>MKTRLEQVLERYLNGREVAVWGVPTRRLLRALKPFKFHTADRVDPQYHYVVAVTDDDLTDFLSDEQSKSFQYANDYLTFDDEGGELPFERMCFNVPVGRQTYFGDGVVGACENGYIKSIGQFTSINGTAEIHANHQLNMTFVSDDIQNFFNEESMAVFQEKLRKDPKHPYAYSKEPMTIGSDVYIGAHAFINASTVTSIGDGAIIGSGAVVLENVPPFAVVVGVPARIKRYRFSKEMIETLLRVKWWDWSIEEINENVDALISPE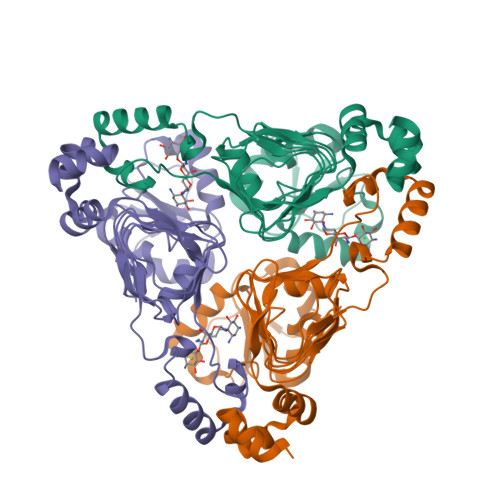LFMKKYGSL[3x]> GSPGIHMNSIKNVPARVLSRRPGHSLEAEREQFDKTQAISISKAINSQEAPVKEKHARRIILGTHHEKGAFTFWSYAIGLPLPSSSILSWKFCHVLHKVLRDGHPNVLHDCQRYRSNIREIGDLWGHLRDQYGHLVNIYTKLLLTKISFHLKHPQFPAGLEVTDEVLEKAAGTDVNNIFQLTVEMFDYMD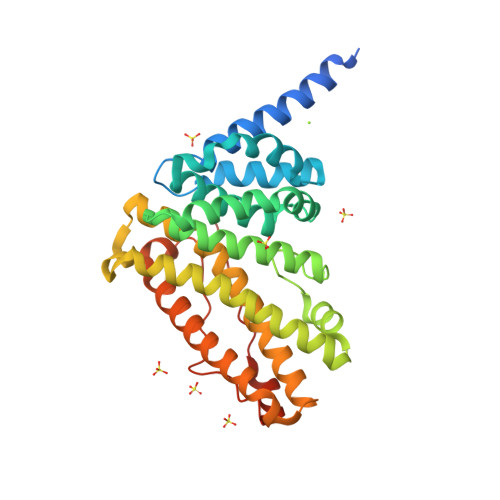CELKLSESVFRQLNTAIAVSQMSSGQCRLAPLIQVIQDCSHLYHYTVKLMFKLHSCLPADTLQGHRDRFHEQFHSLRNFFRRASDMLYFKRLIQIPRLPEGPPNFLRASALAEHIKPVVVIPEEAPEE>[14x]TTTVGLVCKDGVVMATEKRATMGNFIASKAAKKIYQIADRMAMTTAGSVGDAQFLARIIKIEANLYEIRRERKPTVRAIATLTSNLLNSYRYFPYLVQLLIGGIDSEGKSIYSIDPIGGAIEEKDIVATGSGSLTAYGVLEDRFTPEIGVDEAVELAVRAIYSAMKRDSASGDGIDVVKITEDEFYQYSPEEVEQILAKFRK;>QMGYDRAITVFSPDGRLFQVEYAREAVKRGATAIGIKCKEGVILIADKRVGSKLLEADTIEKIYKIDEHICAATSGLVADARVLIDRARIEAQINRLTYDEPITVKELAKKICDFKQQYTQYGGVRPFGVSLLIAGVDEVPKLYETDPSGALLEYKATAIGMGRNAVTEFFEKEYRDDLSFDDAMVLGLVAMGLSIESELVPENIEV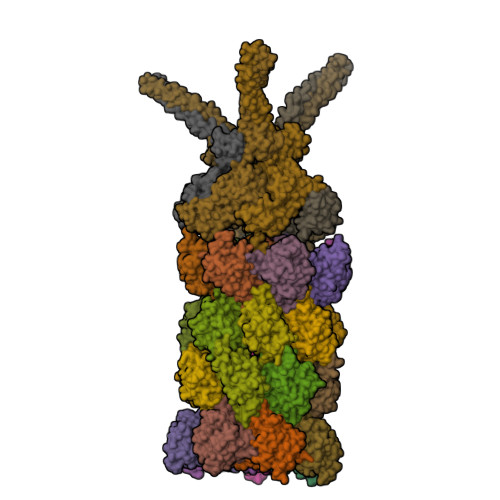GYVKVDDRTFKEVSPEELKPYVERANERIRELLKK[14x];>LLEKLKKLEEDYYKLRELYRRLEDEKKFIESERIRYEREVRRLRSEVERLRSPPLLVGVVSDILEDGRVVVKSSTGPKFVVNTSQYINEEELKPGARVALNQQTLAIVNVLPTSKDPMVYGFEVEEKPEVSYEDIGGLDVQIEEIREAVELPLLKPELFAEVGIEPPKGVLLYGPPGTGKTLLAKAVANQTRATFIRVVGSEFVQKYIGEGARLVREVFQLAKEKAPSIIFIDELDAIAARRTNSDTSGDREVQRTMMQLLAELDGFDPRGDVKVIGATNRIDILDPAILRPGRFDRIIEVPLPTFEGRIQIFKIHTRKMKLAEDVDFKELARITEGASGADIKAICTEAGMFAIREERAKVTMLDFTKAIEKVLKKTTPIPDLKGVMFV[6x]>KLLLANWGLPKAVLEKYHSFGVKKMFEWQAECLLLGQVLEGKNLVYSAPTSAGKTLVAELLILKRVLEMRKKALFILPFVSVAKEKKYYLQSLFQEVGIKVDGYMGSTSPSRHFSSLDIAVCTIERANGLINRLIEENKMDLLGMVVVDELHMLGDSHRGYLLELLLTKICYITRKSASCQADLASSLSNAVQIVGMSATLPNLELVASWLNAELYHTDFRPVPLLESVKVGNSIYDSSMKLVREFEPMLQVKGDEDHVVSLCYETICDNHSVLLFCPSKKWCEKLADIIAREFYNLHHQAEGLVKPSECPPVILEQKELLEVMDQLRRLPSGLDSVLQKTVPWGVAFHHAGLTFEERDIIEGAFRQGLIRVLAATSTLSSGVNLPARRVIIRTPIFGGRPLDILTYKQMVGRAGRKGVDTVGESILICKNSEKSKGIALLQGSLKPVRSCLQRREGEEVTGSMIRAILEIIVGGVASTSQDMHTYAACTFLAASMKEGKQGIQRNQESVQLGAIEACVMWLLENEFIQSTEASDGTEGKVYHPTHLGSATLSSSLSPADTLDIFADLQRAMKGFVLE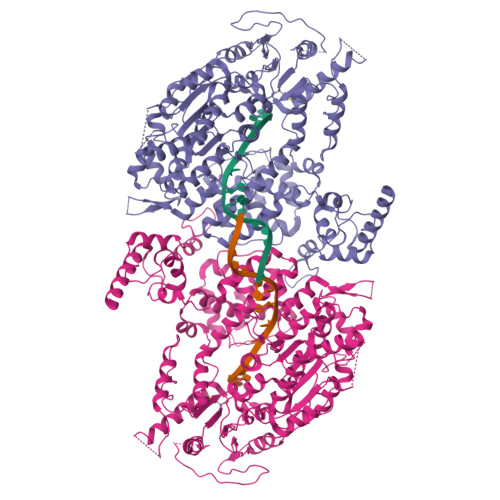NDLHILYLVTPMFEDWTTIDWYRFFCLWEKLPTSMKRVAELVGVEEGFLARCVAAAAAAAAAAQHRQMAIHKRFFTSLVLLDLISEVPLREINQKYGCNRGQIQSLQQSAAVYAGMITVFSNRLGWHNMELLLSQFQKRLTFGIQRELCDLVRVSLLNAQRARVLYASGFHTVADLARANIVEVEVILKNAVPFKSARKAVDEEEEAVEERRNMRTIWVTGRKGLTEREAAALIVEEARMILQQDL[2x]>[4x]QMNYEEVIKKYRGEENFDHAAYDWRLHSGVTPVKDQKNCGSCWAFSSIGSVESQYAIRKNKLITLSEQELVDCSFKNYGCNGGLINNAFEDM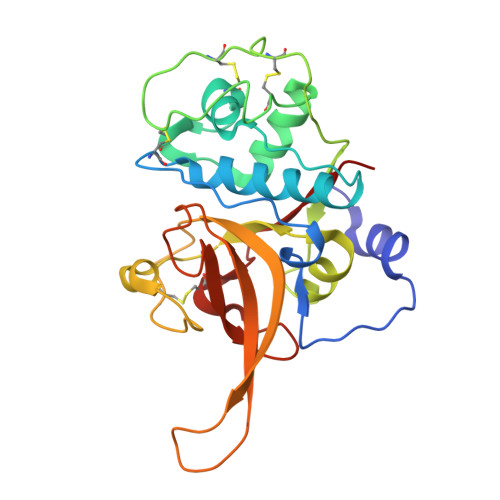IELGGICPDGDYPYVSDAPNLCNIDRCTEKYGIKNYLSVPDNKLKEALRFLGPISISVAVSDDFAFYKEGIFDGECGDQLNHAVMLVGFGMKEIVNPLTKKGEKHYYYIIKNSWGQQWGERGFINIETDESGLMRKCGLGTDAFIPLIE>GAMDMETPSQRRATRSGAQASSTPLSPTRITRLQEKEDLQELNDRLAVYIDRVRSLETENAGLRLRITESEEVVSREVSGIKAAYEAELGDARKTLDSVAKERARLQLELSKVREEFKELKARNTKKEGDLIAAQARLKDLE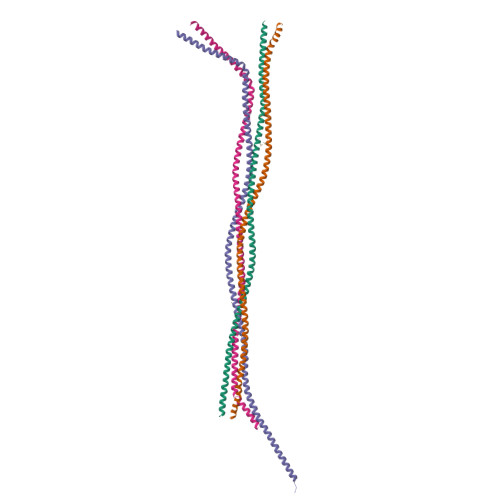ALLNSKEAALSTALSEKRTLEGELHDLRGQVAKLEAALGEAKKQLQDEMLRRVDAENRLQTMKEELDFQKNIYSEELRETKRRHETRLVEIDNGKQREFESRLADALQELRAQHEDQVEQYKKELEKTYSAKLDNARQSAERNSNLVGAAHEELQQSRIRID[4x]>[2x]TPEMPVLENRAAQGNITAPGGARRLTGDQTAALRNSLSDKPAKNIILLIGDGMGDSEITAARNYAEGAGGFFKGIDALPLTGQYTHYALNKKTGKPDYVTDSAASATAWSTGVKTYNGALGVDIHEKDHPTILEMAKAAGLATGNVSTAELQDATPAALVAHVTSRKCYGPSATSQKCPGNALEKGGKGSITEQLLNARADVTLGGGA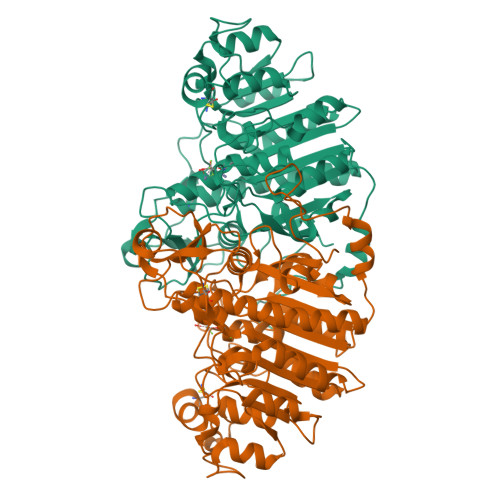KTFAETATAGEWQGKTLREEAEARGYQLVSDAASLNSVTEANQQKPLLGLFADGNMPVRWLGPKATYHGNIDKPAVTCTPNPQRNDSVPTLAQMTDKAIELLSKNEKGFFLQVEGASIDKQNHAANPCGQIGETVDLDEAVQRALEFAKKEGNTLVIVTADHAHASQIVAPDTKAPGLTQALNTKDGAVMVMSYGNSEEDSQEHTGSQLRIAAYGPHAANVVGLTDQTDLFYTMKAALGLK> MNLRAAGPGWLFCPADAPEAFAAAAAAADVVILDLEDGVAEAQKPAARNALRDTPLDPERTVVRINAGGTADQARDLEALAGTAYTTVMLPKAESAAQVIELAPRDVIALVETARGAVCAAEIAAADPTVGMMWGAEDLIATLGGSSSRRADGAYRDVARHVRSTILLAASAFGRLALDAVHLDILDVEGLQEE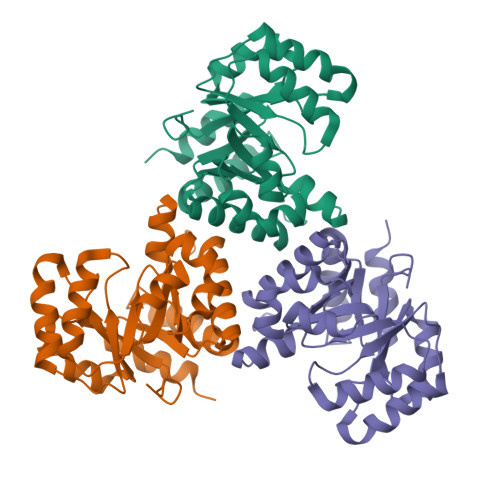ARDAAAVGFDVTVCIHPSQIPVVRKAYAASHEKLAWARRVLAASRSERGAFAFEGQMVDSPVLTHAETMLRRAGEATSE> R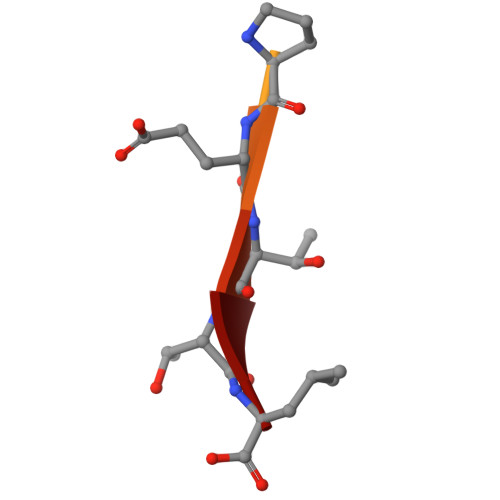RVRKLPETTL> MVDLPVIQPRLCTHARWPAPVYGLLVDPSLPSNPQWQNGRVHVDGTLLGTTPISGSWVSCFAAEAAYKFQSGTGEVATFTLIEQDGSAYVPGDRAAPLGYPDFSGQLEIEVQTETTKTGDKLKVTTFEMILGPTTNADQAPYQGRVFASVTAAASLDLVDGRVRAVPRSIYGFQDTIPEYNDGLLVPLAPPIGPFLPGEVLLRFRTYMRQIDTADAAAEAIDCALPQEFVSW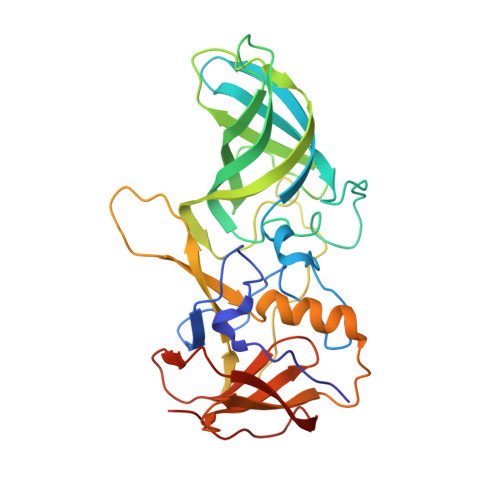FASNAFTVQSEALLLRYRNTLTGQLLFECKLYNEGYIALSYSGSGPLTFPTDGIFEVVSWVPRLYQLASVG LysG detects the basic amino acids l-lysine, l-histidine, and l-arginine and activates gene expression of the amino acid transporter encoding gene lysE in the presence of elevated intracellular amino acid concentrations. LysG is a member of the LysR-type transcriptional regulator (LTTR) family, a large and highly conserved group of TRs ubiquitous in bacteria. LysG shows the typical features of LTTRs, a two-lobed regulatory domain linked to the DNA-binding domain by a flexible loop. Two LysG monomers are coupled by dimerization of their DNA-binding domains, forming a winged helix-turn-helix motif responsible for DNA binding.

Interestingly, all attempts to crystallize LysG in the presence of l-lysine and l-histidine failed, but diffraction datasets could be collected to solve the structure of LysG in the free form [LysG], and together with bound ligand l-arginine [LysG + Arg] at 2.52 Å and 3.00 Å, respectively. The ligand-binding pocket is formed by the interface of the two lobes of the regulatory domain. Binding of l-arginine in the extended protomer of [LysG + Arg] leads to a small but substantial tilt of helix 6 by 8° compared to the conformation in the ligand-free protomer [LysG], which enables coordination of the ligand l-arginine by amino acid residues D124 and E125 in the [LysG + Arg] structure. Within the ligand-binding cavity of the [LysG + Arg] structure, sidechains of eight residues (N95, D97, D124, E125, H161, F189, D193, and F222) are located within a distance of <3.6 Å to the bound l-arginine molecule, potentially interacting with this effector molecule and the other two basic amino acids. However, since no diffracting LysG crystals in the presence of l-lysine or l-histidine could be obtained, blind docking calculations using the [LysG + Arg] structure and AutoDock Vina21 were performed, which predicted the positions of l-arginine, l-lysine, and l-histidine to be in the same binding pocket, with a maximum center of mass deviation of the top ten docking poses from the crystal l-arginine of 1.2 Å, 1.2 Å, and 1.3 Å, respectively. Two 1 µs simulations of LysG revealed two frequently occupied conformations with a reaction coordinate that can be exactly described by the distance between Cα atoms of residues 219 and 96, which are 6.4 Å apart in the effector-occupied (closed) RD in the LysG-Arg structure. Simulation of l-arginine in the ligand-binding site of both TRs yielded no transitions from closed to open conformation on the sub microsecond timescale when started from the crystal structure. Perturbation of the l-arginine orientation by 180-degree rotation resulted in an opening of the conformation, and a subsequent reorientation of l-arginine into the crystal structure orientation for both TRs.

>[2x]MNPIQLDTLLSIIDEGSFEGASLALSISPSAVSQRVKALEHHVGRVLVSRTQPAKATEAGEVLVQAARKMVLLQAETKAQLSGRLAEIPLTIAINADSLSTWFPPVFNEVASWGGATLTLRLEDEAHTLSLLRRGDVLGAVTREANPVAGCEVVELGTMRHLAIATPSLRDAYMVDGKLDWAAMPVLRFGPKDVLQDRDLDGRVDGPVGRRRVSIVPSAEGFGEAIRRGLGWGLLPETQAAPMLKAGEVILLDEIPIDTPMYWQRWRLESRSLARLTDAVVDAAIEGLRP> MSNHSSDIEVGHSMNLTNHFLVAMPSMKDPYFKRSVIYICEHNQDGAMGLMINAPIDITVGGMLKQVDIEPAYPQSHQENLKKPVFNGGPVSEDRGFILHRPRDHYESSMKM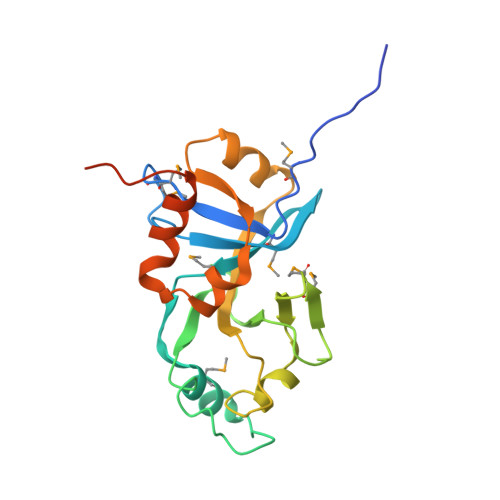TDDIAVTTSKDILTVLGTEAEPEGYIVALGYSGWSAGQLEVELTENSWLTIEADPELIFNTPVHEKWQKAIQKLGISPAQLSSDAGHALEHHHHHH>SNAMSTTFAARLNRLFDTVYPPGRGPHTSAEVIAALKAEGITMSAPYLSQLRSGNRTNPSGATMAAL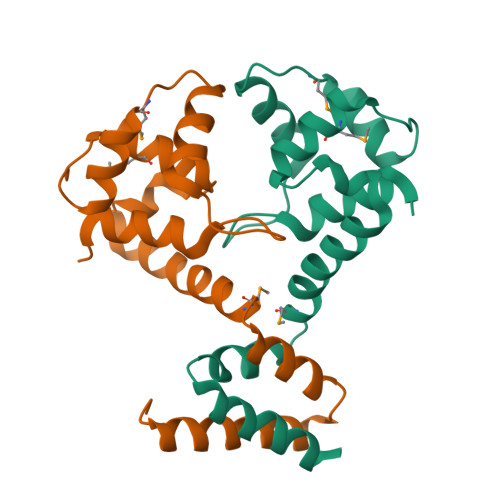ANFFRIKAAYFTDDEYYEKLDKELQWLCTMRDDGVRRIAQRAHGLPSAAQQKVLDRIDELRRAEGIDA[18x]> GGAHMDAPMEDAPAPVAQVKVIFTTTEPDLELPESKRQLLVPADIRRYGLSRILNSESMLDTGSIPFDFLINGSFLRSSLEDYLTSNGLSLETTLTLQYVRSLIPPVYEASFEHDDWVSAVDVLSATSPAGRWSSAANSSAAVQPGQERVLSASYDGLLRIW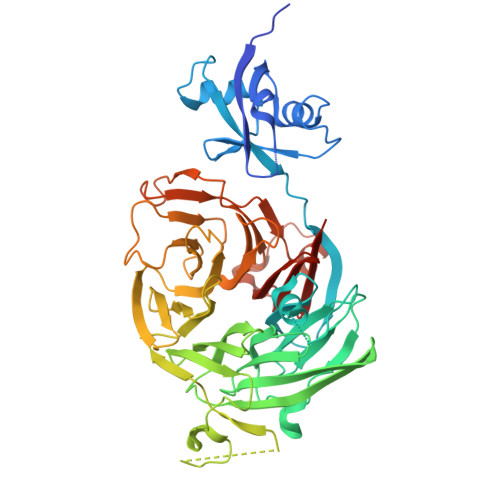NASGSVIATSPSGSHGGHTASIKAAKFLTSDRLASAGMDRTVRVWKYTESDHFTGELKPTLELYGHTGSVDWLDVDGHSKHILTASADGAIGFWSASKASAPEPDASLLPGAHVSKRRKATSSVSTAQRGPLGLWSIHTAPATAAIFDPRDRTVAYSASQDHTVRTLDLTTGQVVSTLTLTHPLLSLSALTRAGTTSPLLAAGTSARHITMVDPRASSATTSVMTLRGHANKVVSLSPSPENEYSLVSGSHDGTCRVWDLRSVRPATKEEGSLGGVSEPVYVIERESWASKGKKKRPVAGDGCKVFSVVWDKLGIFSGGEDKKVQVNRGRNIVTEQK> MEFIMKTRMFEEEGWIRKKCKVCGKPFWTLDPDRETCGDPPCDEYQFIGKPGIPRKYTLDEMREKFLRFFEKHEIYPHGRVKRYPVLPRWRDDVLLVGASIMDFQPWVISGEADPPANPLVISQPSIRFTDIDNVGITGRHFTIFEMMAHHAFNYPGKPIYWMDETVELAFEFFTKELKMKPEDITFKENPWAGGGNAGPAFEVLYRGLEVATLVFMQYKKAPENAPQDQVVVIKGEKYIPMETKVVDTGYGLERLVWMSQGTPTAYDAVLGYVVEPLKKMAGIEKIDEKILMENSRLAGMFDIEDLGDLRYLREQVAKRVGITVEELEKAIRPYELIYAIADHTKALTFMLADGVVPSNVKAGYLARLLIRKSIRHLRELGLEVPLSEIVALHIKELHKTFPEFKEMEDIILEMIELEEKKYAETLRRGSDLVRREIAKLKKKGIKEIPVEKLVTFYESHGLTPEIVKEIAEKEGVKVNIPDNFYSMVAKEAERTKEEKGEELVDFELLKDLPDTRRLYYEDPFMKEFDAKVLRVIKDWVILDAT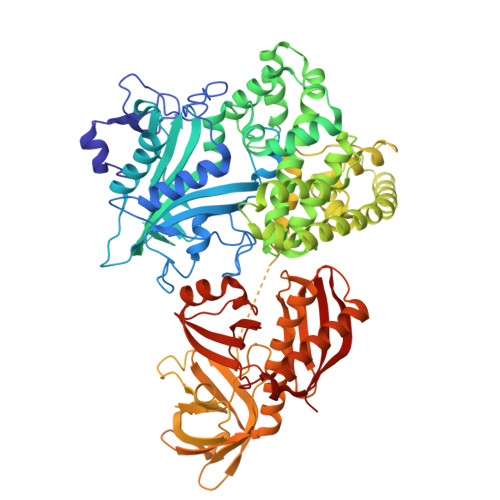AFYPEGGGQPYDTGVLIVNGREVKVTNVQKVGKVIIHKVEDPGAFKEGMIVHGKIDWKRRIQHMRHHTGTHVLMGALVRVLGRHVWQAGSQLTTDWARLDISHYKRISEEELKEIEMLANRIVMEDRKVTWEWLPRTTAEQKYGFRLYQGGVVPGREIRVVKIEDWDVQACGGTHLPSTGLVGPIKILRTERIQDGVERIIFACGE>[60x]MWRVCARRAQNAAPRAGFGARWTALREEPGAPCAAPRAGSVPARCSSTTRGYGRSRALCGWSASSWATPQNRILLQLWGSPNRRWYSLPPHQKVPLPSLSPTMQAGTIARWEKKEGDKINEGELIAEV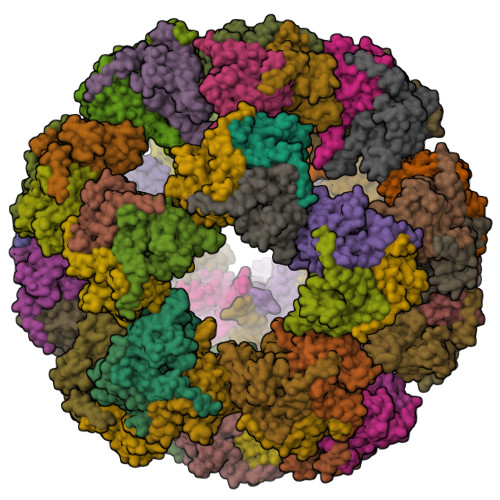ETDKATVGFESLEECYMAKILVAEGTRDVPVGAIICITVEKPEDIEAFKNYTLDSSAAPAPQAAPAPTPAAAAPAPTPSAQAPGSSYPTHMQVVLPALSPTMTMGTVQRWEKKVGEKLSEGDLLAEIETDKATIGFEVQEEGYLAKILIPEGTRDVPLGTPLCIIVEKEADIPAFADYRPTEVTDLKPPAPPPTPSPVTPVPPAPQPVAPTPAATRPATPAGPKGRLFVSPLAKKLASEKGIDLTQIKGTGPDGRIIKKDIDSFVPTKAAPTPAAAVPPPSPGVAPVPTGVFTDIPISNIRRVIAQRLMQSKQTIPHYYLSVDVNMGEVLLVRKELNKMLEGRSKISVNDFIIKASALACLKVPEANSSWLDTVIRQNHVVDISVAVSTPAGLITPIVFNAHIKGLETIANDVVSLATKAREGKLQPHEFQGGTFTISNLGMFGIKNFSAIINPPQACILAVGASEDRLFPADNEKGFDVASMMSVTLSCDHRVVDGAVGAQWLAEFRKYLEKPITMLL N-{4-[5-(phenanthren-2-yl)-3-(trifluoromethyl)-1H-pyrazol-1-yl]phenyl}glycinamide | C26 H19 F3 N4 O | 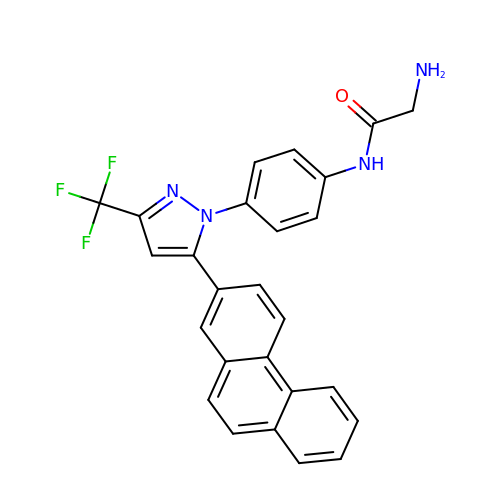YULUCECVQOCQFQ-UHFFFAOYSA-N6-AMINO-3,9-DIMETHYL-9H-PURIN-3-IUM | C7 H10 N5 | 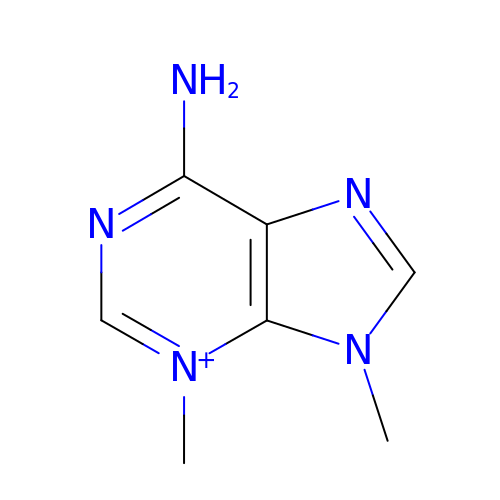YXTNRNJPEDJTNF-UHFFFAOYSA-O> MRLLVTGGAGFIGSHFVRQLLAGAYPDVPADEVIVLDSLTYAGNRANLAPVDADPRLRFVHGDIRDAGLLARELRGVDAIVHFAAESHVDRSIAGASVFTETNVQGTQTLLQCAVDAGVGRVVHVSTDEVYGSIDSGSWTESSPLEPNSPYAASKAGSDLVARAYHRTYGLDVRITRCCNNYGPYQHPEKLIPLFVTNLLDGGTLPLYGDGANVREWVHTDDHCRGIALVLAGGRAGEIYHIGGGLELTNRELTGILLDSLGADWSSVRK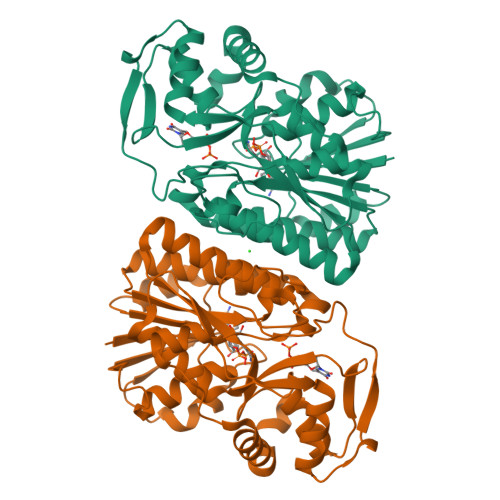VADRKGHDLRYSLDGGKIERELGYRPQVSFADGLARTVRWYRENRGWWEPLKATAPQLPATAVEVSA>MDVNDNEPIFVSSPFQATVLENVPLGYPVVHIQAVDADSGENARLHYRLVDTASTFLGGGSAGPKNPAPTPDFPFQIHNSSGWITVCAELDREEVEHYSFGVEAVDHGSPPMSSSTSVSITVLDVNDNDPVFTQPTYELRLNEDAAVGSSVLTLQARDRDANSVITYQLTGGNTRNRFALSSQRGGGLITLALPLDYKQEQQYVLAVTASDGTRSHTAHVLINVTDANTHRPVFQSSHYT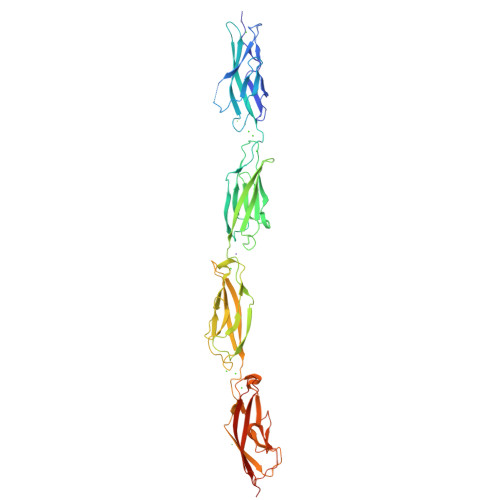VSVSEDRPVGTSIATLSANDEDTGENARITYVIQDPVPQFRIDPDSGTMYTMMELDYENQVAYTLTIMAQDNGIPQKSDTTTLEILILDANDNAPQFLWDFYQGSIFEDAPPSTSILQVSATDRDSGPNGRLLYTFQGGDDGDGDFYIEPTSGVIRTQRRLDRENVAVYNLWALAVDRGSPTPLSASVEIQVTILDINDNALEHHHHHH[2x]>[3x]MAKEKARYFTFLLYPESIPSDWELKLET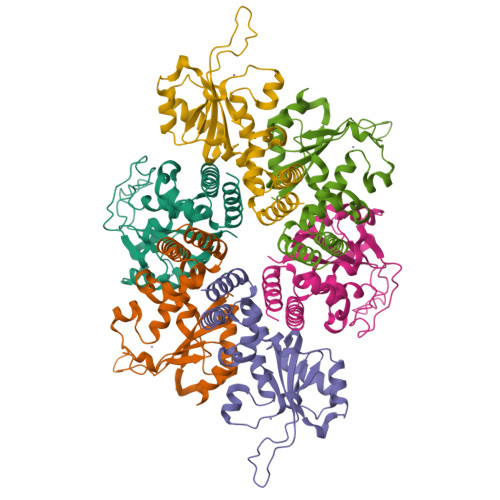LGVPMAISPLHDKDKSSIKGQKYKKAHYHVLYIAKNPVTADSVRKKIKLLLGEKSLAMVQVVLNVENMYLYLTHESKDAIAKKKHVYDKADIKLINNFDIDRYVTLDVEEKTELFNVVVSLIRAYTLQNIFDLYDFIDENGETYGLTINLVNEVIAGKTGFMKLLFDGAYQRSKRGTKNEER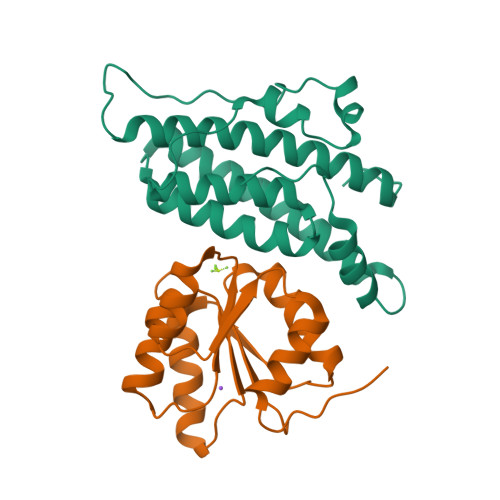> MSTIPSEIINWTILNEIISMDDDDSDFSKGLIIQFIDQAQTTFAQMQRQLDGEKNLTELDNLGHFLKGSSAALGLQRIAWVCERIQNLGRKMEHFFPNKTELVNTLSDKSIINGINIDEDDEEIKIQVDDKDENSIYLILIAKALNQSRLEFKLARIELSKYYNTNL;> TSVKILVVEDNHVNQEVIKRMLNLEGIENIELACDGQEAFDKVKELTSKGENYNMIFMDVQMPKVDGLLSTKMIRRDLGYTSPIVALTAFADDSNIKECLESGMNGFLSKPIKRPKLKTILTEFCAAYQGKKN>[6x]FGSICAFTASRTFPNGFTVTEEFADADPIDSPPFAAADTGAGLNGDMVVWNRANILEVVVNVIPNTEGERNLAVLLDANRTGKDKSGARDVVGLVVAMPDGSKITCTNGTPIDGVLINAVASVGRLKTKPYRFRFEKVIKAGTS;> MISQSRYIRIISGVGAAAPVAGRKLILRVMTTNNVIPPGIVIEFDNANAVLSYFGAQSEEYQRAAAYFKFISKSVNSPSSISFARWVNTAIAPMVVGDNLPKTIADFAGFSAGVLTIMVGAAEQNITAIDTSAATSMDNVASIIQTEIRKNADPQLAQATVTWNQNTNQFTLVGATIGTGVLAVAKSADPQDMSTALGWSTSNVVNVAGQSADLPDAAVAKSTNVSNNFGSFLFAGAPLDNDQIKAVSAWNAAQNNQFIYTVATSLANLGTLFTLVNGNAGTALNVLSATAANDFVEQCPSEILAATNYDEPGASQNYMYYQFPGRNITVSDDTVANTVDKSRGNYIGVTQANGQQLAFYQRGILCGGPTDAVDMNVYANEIWLKSAIAQALLDLFLNVNAVPASSTGEAMTLAVLQPVLDKATANGTFTYGKEISAVQQQYITQVTGDRRAWRQVQTLGYWINITFSSYTNSNTGLTEWKANYTLIYSKGDAIRFVEGSDVMI

Bacteriophage E217 infects Pseudomonas aeruginosa and is part of an experimental phage cocktail developed to eradicate P. aeruginosa infections in Galleria mellonella (wax moth) larvae and vertebrate models. E217 is a PB1-like Myoviridae of the Pbunavirus genus characterized by a ~66.2 kbp genome, significantly smaller than the classical enterobacteria phage T4 (~169 kbp). Here, we describe the structure of the whole E217 virion before and after DNA ejection at 3.1 Å and 4.5 Å resolution, respectively, determined using cryogenic electron microscopy (cryo-EM). We identify and build de novo structures for 19 unique E217 gene products, resolve the tail genome-ejection machine in both extended and contracted states, and decipher the complete architecture of the baseplate formed by 66 polypeptide chains.

We determined cryo-EM reconstructions of the extended and contracted E217 sheath at 3.1 Å resolution (FSC = 0.143). At the quaternary structure level, the extended conformation of the E217 sheath consists of a helical tube of ~205 Å in diameter that has a regular pitch of 490 Å and rise and twist of 40.8 Å and 31.3°, respectively. The extended sheath is porous, with visible openings between subunits. The internal lumen is ~75 Å and houses the tail tube (described in the next section). Stacked hexamers of the tail tube protein gp32 form the central tube of the E217 tail. Six copies of gp32 assemble laterally to form a hollow hexamer, whose internal lumen measures ~40 Å in diameter. The interface between gp32 subunits is stabilized by 11 hydrogen bonds, many of which form between residues exposed by the extended β-turn. The interior surface of the tube is mildly charged, with two charged patches, one positive, exposed by Arg125/Lys127, and the other negative, formed by Asp27. Before genome ejection, each tail tube subunit contacts one sheath protein generating an extensive interaction surface stabilized by two hydrogen bonds, one salt bridge, and 99 van der Waals contacts. Notably, tail sheath subunits do not contact each other in the extended tail but are solely connected by the association of their C-terminal β-turns and N-/C-terminal arms.> AGSSMASANLEGDALHTLRVTLVDPNNVLQSWDPTLVNPCTWFHVTCNNENSVIRVDLGNAELSGHLVPELGVLKNLQYLELYSNNITGPIPSNLGDLTNLVSLDLYLNSFSGPIPESLGKLSKLRFLRLNNNSLTGSIPMSLT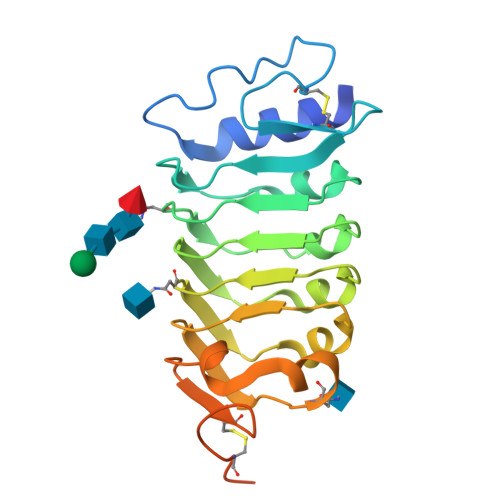QITTLQVLDLSNNRLSGSVPDNGSFSLFTPISFANNLDLCGPVTSHPCPGSLENLYFQGAWSHPQFEKGSHHHHHHHHH>[2x]GHMPNIPPPFTAPYAPDDAEIAARLLPASHLSPPQEARIHRTATRLIEAIRKRDDRLGGVEDMLREFALSTKEGLALMVLAEALLRVPDARTADQFIEDKLGEGDFIHHETKSTAFLVNASAWALGLSARVIQPGETPDGTIGRLVKRLGAPAVRTATRQAMRLMGNHFVLGETIEQALERGKPRSGQKTRYSFDMLGEGARTAADARRYFDAYASAIETIGKAAGNHALPDRPGISVKLSALHPRFEAISRARVMVELVPQLLDLAQRAKAHDLNFTVDAEEADRLELSLDVIAATLADPSLKGWDGFGLAIQAYQKRASAVIDYV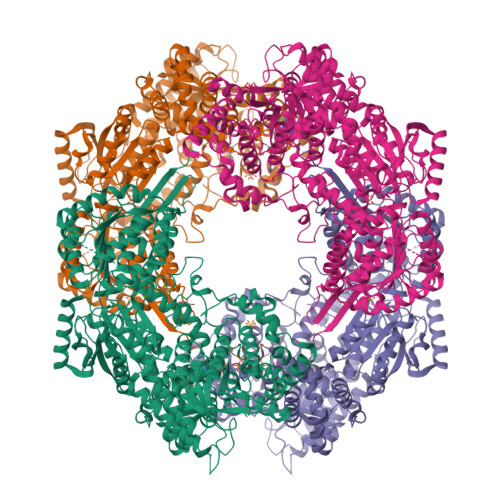DALARAHDRKLMVRLVKGAYWDTEIKRAQERGLDGYPVFTRKAMTDLNYVACASKLLALRPRIFPQFATHNALTVATVLEMAEGSSGFEFQRLHGMGEALYEQLAKDHADIAYRTYAPVGSHRDLLAYLVRRLLENGANSSFVAQAADYRVPVPALLQRPADAIVRPQAAAHPRIPLPCDLFAPERRNSRGVEFGARTALDQLLTDVKAETGDLKPIADATPDQAHAAVAAARAGFAGWSRTPAGIRAAALEQAAHLLESRSAHFIALLQREGGKTLDDALSELREAADFCRYYAAQGRKLFGSETAMPGPTGESNALTMRGRGVFVAISPWNFPLAIFLGQVTAALMAGNSVVAKPAEQTPRIAREAVALLHEAGIPKSALYLVTGDGRIGAALTAHPDIAGVVFTGSTEVARSINRALAAKDGPIVPLIAETGGINAMIADATALPEQVADYVVTSAFRSAGQRCSALRLLFVQEDVADRMIEMVAGAARELKIGDPSDVATHVGPVIDVEAKQRLDAHIARMKTEARLHFAGPAPEGCFVAPHIFELTEAGQLTEEVFGPILHVVRYRPENLERVLRAIERTGYGLTLGVHSRIDDSIEAIIDRVQVGNIYVNRNMIGAVVGVQPFGGNGLSGTGPKAGGPHYLARFATEQTVTINTAAAGGNAALLAGEE> MKRIPRKTKGKSSGKGNDSTERADDGSSQLRDKQNNKAGPATTEPGTSNREQYKARPGIASVQRATESAEMPMKNNDEGTPDKKGNTKGDLVNEHSEAKDEADEATKKQAKDTDKSKAQVTYSDTGINNANELSRSGNVDNEGGSNQKPMSTRIAEATSAIVSKHPARVGLPPTASSGHGYQCHVCSAVLFSPLDLDAHVASHGLHGNMTLTSSDIQRHITEFISSWQNHPIVQVSADVENKKTAQLLHADTPRLVTWDAGLCTSFKIVPIVPAQVPQDVLAYTFFTSSYAIQSPFPEAAVSRIVVHTRWASNVDFDRDSSVIMAPPTENNIHLFKQLLNTETLSVRGANPLMFRANVLHMLLEFVLDNLYLNRHTGFSQDHTPFTEGANLRSLPGPDAEKWYSIMYPTRMGTPNVSKICNFVASCVRNRVGRFDRAQMMNGAMSEWVDVFETSDALTVSIRGRWMARLARMNINPTEIEWALTECAQGYVTV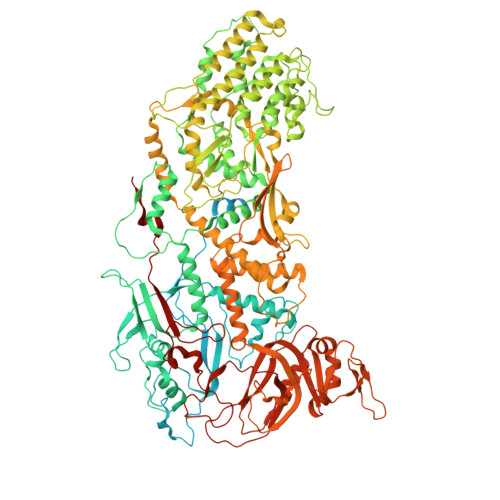TSPYAPSVNRLMPYRISNAERQISQIIRIMNIGNNATVIQPVLQDISVLLQRISPLQIDPTIISNTMSTVSESTTQTLSPASSILGKLRPSNSDFSSFRVALAGWLYNGVVTTVIDDSSYPKDGGSVTSLENLWDFFILALALPLTTDPCAPVKAFMTLANMMVGFETIPMDNQIYTQSRRASAFSTPHTWPRCFMNIQLISPIDAPILRQWAEIIHRYWPNPSQIRYGAPNVFGSANLFTPPEVLLLPIDHQPANVTTPTLDFTNELTNWRARVCELMKNLVDNQRYQPGWTQSLVSSMRGTLDKLKLIKSMTPMYLQQLAPVELAVIAPMLPFPPFQVPYVRLDRDRVPTMVGVTRQSRDTITQPALSLSTTNTTVGVPLALDARAITVALLSGKYPPDLVTNVWYADAIYPMYADTEVFSNLQRDMITCEAVQTLVTLVAQISETQYPVDRYLDWIPSLRASAATAATFAEWVNTSMKTAFDLSDMLLEPLLSGDPRMTQLAIQYQQYNGRTFNIIPEMPGSVIADCVQLTAEVFNHEYNLFGIARGDIIIGRVQSTHLWSPLAPPPDLVFDRDTPGVHIFGRDCRISFGMNGAAPMIRDETGLMVPFEGNWIFPLALWQMNTRYFNQQFDAWIKTGELRIRIEMGAYPYMLHYYDPRQYANAWNLTSAWLEEITPTSIPSVPFMVPISSDHDISSAPAVQYIISTEYNDRSLFCTNSSSPQTIAGPDKHIPVERYNILTNPDAPPTQIQLPEVVDLYNVVTRYAYETPPITAVVMGVP Human aromatic amino acid decarboxylase (AADC) is a pyridoxal 5′‐phosphate‐dependent enzyme responsible for the biosynthesis of dopamine and serotonin, essential neurotransmitters involved in motor and cognitive abilities. Mutations in its gene lead to AADC deficiency, a monogenic rare neurometabolic childhood parkinsonism characterized by severe motor and neurodevelopmental symptoms. Here, for the first time, we solved the crystal structure of human holoAADC in the internal aldimine (1.9 Å) and in the external aldimine (2.4 Å) of the substrate analog L‐Dopa methylester. By combining various high‐ and low‐resolution structural approaches, we determined that AADC is a mobile homodimer presenting asymmetric behavior among subunits, thus behaving as a conformational heterodimer.

The superposition of the active sites of human native and DME‐bound AADC shows that the pyridine ring of PLP faintly tilts when it converts from the internal to the external aldimine, being the main difference associated to the presence of the CL from the neighboring subunit orienting the catalytic Tyr332' (the prime denotes residues belonging to the neighboring subunit) in a H‐bond relay with His192 and Ser193 in the proximity to the a‐C of the ligand. Slight changes are observed in the orientation of loop3 residues Arg347' and Leu353' contributing in trans to the active site in the transition from internal to external aldimine. Besides these local changes, further small alterations far from the active site are observed by monitoring the root mean square deviation (RMSD) between native and DME‐bound AADC structures. The highest deviations are observed for loop3 (since it is solved only in the DME‐bound AADC). Slight changes are also visible in the backbone of residues 34–36 belonging to the α1‐loop‐α2 motif (NTD), in the stretch containing residues 434–436, immediately after helix α16 (417–430) and participating to sheet β10 (436–440) (CTD), as well as in the segment 135–139. Crystallographic data of human apo and holoAADC show that Arg27 is placed at the end of helix α1 and interacts with Glu61 of helix α3 through the formation of a salt‐bridge. This saline interaction could favor the assembly of the NTD and in the meanwhile it could properly orient the stretch of the residues 28–36 towards elements of the CTD (the nearby helix α16 close to sheet β10), in turn connected to the active site. Gln28 interacts with Asp32 which is engaged with Lys431 of the CTD, thus reinforcing the network of interactions between NTD and CTD. As for the holo form, the equilibrated structure does not show important divergence in comparison to the crystal structure, even if some small changes are visible in close proximity to helix α6, as in the apo structure. On the contrary, CL flexibility is minimally affected by PLP binding since it is similarly digested in both apo and holo conformations.

> MNASEFRRRGKEMVDYVANYMEGIEGRQVYPDVEPGYLRPLIPAAAPQEPDTFEDIINDVEKIIMPGVTHWHSPYFFAYFPTASSYPAMLADMLCGAIGCIGFSWAASPACTELETVMMDWLGKMLELPKAFLNEKAGEGGGVIQGSASEATLVALLAARTKVIHRLQAASPELTQAAIMEKLVAYSSDQAHSSVERAGLIGGVKLKAIPSDGNFAMRASALQEALERDKAAGLIPFFMVATLGTTTCCSFDNLLEVGPICNKEDIWLHVDAAYAGSAFICPEFRHLLNGVEFADSFNFNPHKWLLVNFDCSAMWVKKRTDLTGAFRLDPTYLKHSHQDSGLITDYRHWQIPLGRRFRSLKMWFVFRMYGVKGLQAYIRKHVQLSHEFESLVRQDPRFEICVEVILGLVCFRLKGSNKVNEALLQRINSAKKIHLVPCHLRDKFVLRFAICSRTVESAHVQRAWEHIKELAADVLRAERE> MELTDEEASFLTRRQLLALSENGDLPDDIEYEVDLDLKFANNRLKRAYIALQAWKKAFYSDPFNTAANWVGPDVCSYKGVFCAPALDDPSVLVVAGIDLNHADIFGYLPPELGLLTDVALFHVNSNRFCGVIPKSLSKLTLMYEFDVSNNRFVGPFPTVALSWPSLKFLDIRYNDFEGKLPPEIFDKDLDAIFLNNNRFESTIPETIGKSTASVVTFAHNKFSGCIPKTIGQMKNLNEIVFIGNNLSGCLPNEIGSLNNVTVFDASSNGFVGSLPSTLSGLANVEQMDFSYNKFTG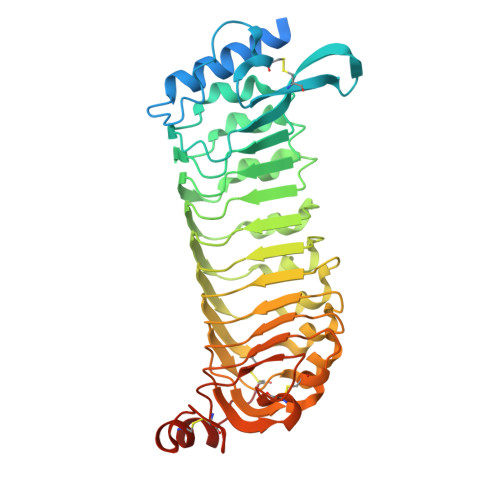FVTDNICKLPKLSNFTFSYNFFNGEAQSCVPGSSQEKQFDDTSNCLQNRPNQKSAKECLPVVSRPVDCSKDKCAGG> SNAFSLKTMSPQNTKATNLIAKARYLRKDEGSNKQVYSVPHFFLAGAAKERSQMNSQTEDHALAPVRNTIQLPTQPLNSEEWDKLKEDLKENTGKTSFESWIISQMAG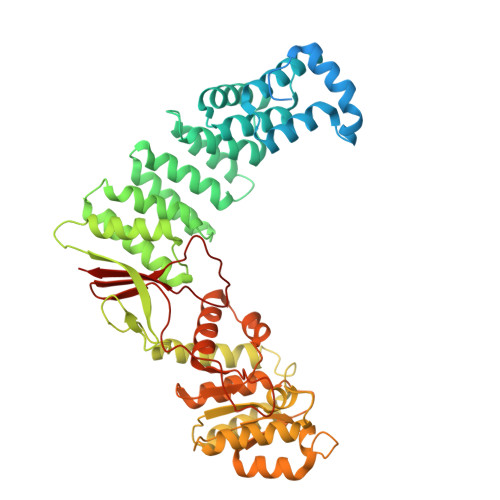CHSSIDVAKSLLAWVAAKNNGIVSYDLLVKYLYLCVFHMQTSEVIDVFEIMKARYKTLEPRGYSLLIRGLIHSDRWREALLLLEDIKKVITPSKKNYNDCIQGALLHQDVNTAWNLYQELLGHDIVPMLETLKAFFDFGKDIKDDNYSNKLLDILSYLRNNQLYPGESFAHSIKTWFESVPGKQWKGQFTTVRKSGQCSGCGKTIESIQLSPEEYECLKGKIMRDVIDGGDQYRKTTPQELKRFENFIKSRPPFDVVIDGLNVAKMFPKVRESQLLLNVVSQLAKRNLRLLVLGRKHMLRRSSQWSRDEMEEVQKQASCFFADDISEDDPFLLYATLHSGNHCRFITRDLMRDHKACLPDAKTQRLFFKWQQGHQLAIVNRFPGSKLTFQRILSYDTVVQTTGDSWHIPYDEDLVERCSCEVPTKWLCLHQKT>[2x]MTMITPSLHQFPGLANKTYFNFGGQGILPTVALEAITAMYGYLQENGPFSIAANQHIQQLIAQLRQALAETFNVDPNTITITDNVTTGCDIVLWGLDWHQGDEILLTDCEHPGIIAIVQAIAARFGITYRFFPVAATLNQGDAAAVLANHLGPKTRLVILSHLLWNTGQVLPLAEIMAVCRRHQGNYPVRVLVDGAQSAGSLPLDFSRLEVDYYAFTGH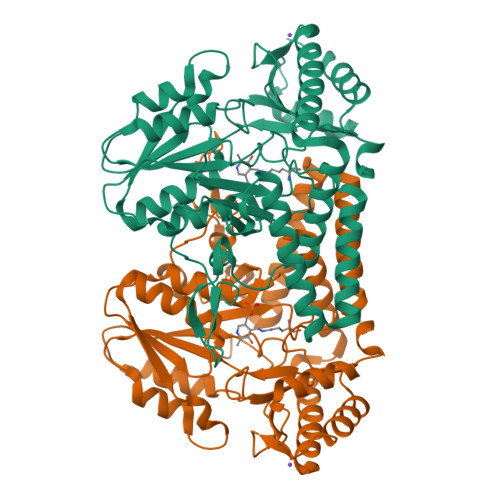KWFAGPAGVGGLYIHGDCLGEINPTYVGWRSITYGAKGEPTGWAEGGKRFEVATSAYPQYAGLLAALQLHQRQGTAEERYQAICQRSEFLWRGLNQLPHVHCLATSAPQAGLVSFTVDSPLGHRAIVQKLEEQRIYLRTIADPDCIRACCHYITDEEEINHLLARLADFGP>GPLGSMPGEEEERAFLVAREELASALRRDSGQAFSLEQLRPLLASSLPLAARYLQLDAARLVRCNAHGEPRNYLNTLSTALNILEKYGRNLLSPQRPRYWRGVKFNNPVFRSTVDAVQGGRDVLRLYGYTEEQPDGLSFPEGQEEPDEHQVATVTLEVLLLRTELSLLLQNTHPRQQALEQLLE[2x]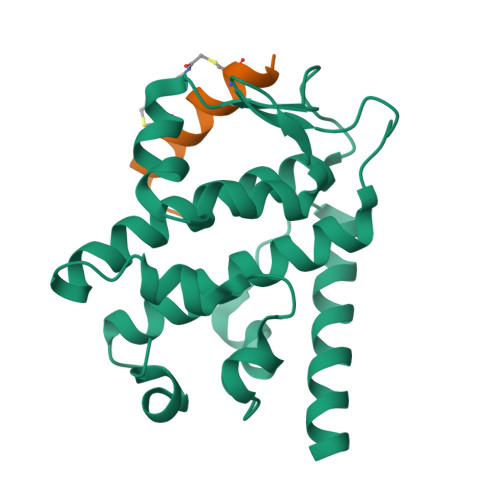;>[2x]DPAIVQCAWAALYCDMQ> ACDYTCGSNCYSSSDVSTAQAAGYKLHEDGETVGSNSYPHKYNNYEGFDFSVSSPYYEWPILSSGDVYSGGSPGADRVVFNENNQLAGSITHTGAS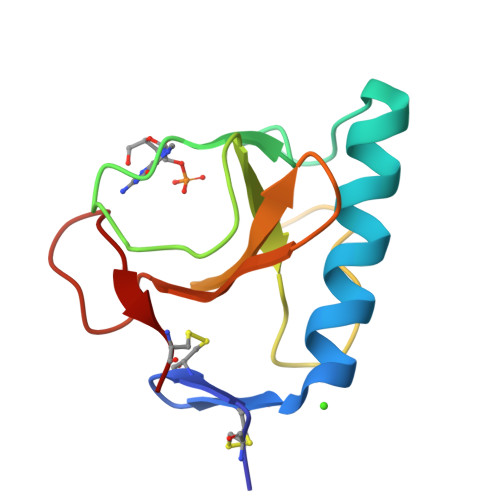GNNFVECT> MTLVPDLTATDLARHRWLTDNSWTRPTWTVAELEAAKAGRTISVVLPALNEEETVGGVVETIRPLLGGLVDELIVLDSGSTDDTEIRAMAAGARVISREVALPEVAPQPGKGEVLWRSLAATTGDIIVF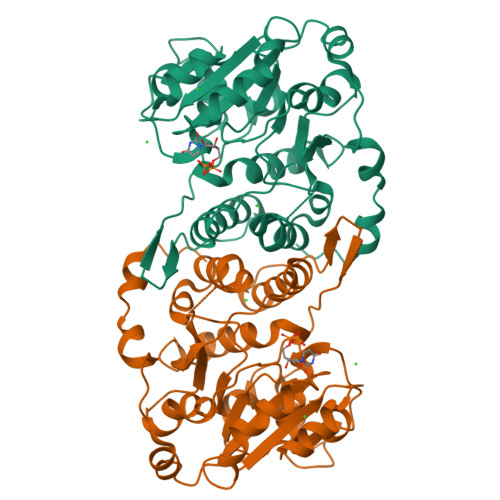IDSDLIDPDPMFVPKLVGPLLLSEGVHLVKGFYRRPLKTSGSEDAHGGGRVTELVARPLLAALRPELTCVLQPLGGEYAGTRELLMSVPFAPGYGVEIGLLVDTYDRLGLDAIAQVNLGVRAHRNRPLTDLAAMSRQVIATLFSRCGVPDSGVGLTQFFADGDGFSPRTSEVSLVDRPPMNTLRGKLAAALEHHHHH Glycerol is metabolized via coupled oxidative and reductive pathways, with glycerol dehydrogenase (GDH; EC 1.1.1.6) serving as the initiator enzyme for the oxidative pathway. GDH catalyzes the oxidation of glycerol to dihydroxyacetone (DHA) with concomitant reduction of NAD+ to NADH. As a member of the family III metal-containing polyol dehydrogenases, GDH requires not only NAD+, but also a metal ion, typically Zn2+, for its activity. The structure of GDH features two well-separated domains, the N- and C-domains; between them is a central cleft where the active site is located.

Full-length E. coli GDH (1–367) was crystallized in the presence of NAD+ and then soaked in glycerol-containing solution for 1 h before flash-freezing in liquid nitrogen for data collection. Within the asymmetric unit of the GDHNAD∙Gly structure, there were two molecules (Mol-A and Mol-B) related by a 2-fold non-crystallographic symmetry. Mol-A formed a ternary complex with both ligands bound at the active site. The binding mode of NAD+ was consistent with previously reported observations, and glycerol coordinated with Zn2+ through its C1-OH oxygen in a non-productive manner or was positioned at a secondary binding site. By contrast, Mol-B had only NAD+ bound without glycerol, and the binding was at an alternative site along the central cleft. It appears that one of the intermediate states in NAD+ access or release was captured. The pH under the crystallization conditions was 4.2, significantly lower than the optimum pH of approximately 10.0 for the forward enzymatic reaction of GDH. Despite the two protomers adopting distinct ligand-bound states, the present GDHNAD∙Gly structure also adopted an octameric structure through crystallographic 4-fold symmetry. Our size-exclusion chromatography experiment, conducted using a HiLoad 16/600 Superdex 200 prep grade column with 50 mM HEPES-NaOH buffer (pH 7.5), also revealed a protein peak corresponding to GDH at a size consistent with its octamer. This octamerization entailed formation of three interfaces per protomer: Interface-1 in the N-domain and Interfaces-2 and -3 in the C-domain. Accordingly, each protomer of the GDH octamer could independently bind ligands, as was observed in the GDHNAD∙Gly structure.

>[2x]MDRIIQSPGKYIQGADVINRLGEYLKPLAERWLVVGDKFVLGFAQSTVEKSFKDAGLVVEIAPFGGECSQNEIDRLRGIAETAQCGAILGIGGGKTLDTAKALAHFMGVPVAIAPTIASTDAPCSALSVIYTDEGEFDRYLLLPNNPNMVIVDTKIVAGAPARLLAAGIGDALATWFEARACSRSGATTMAGGKCTQAALALAELCYNTLLEEGEKAMLAAEQHVVTPALERVIEANTYLSGVGFESGGLAAAHAVHNGLTAIPDAHHYYHGEKVAFGTLTQLVLENAPVEEIETVAALSHAVGLPITLAQLDIKEDVPAKMRIVAEAACAEGETIHNMPGGATPDQVYAALLVADQYGQRFLQEWELEHHHHHH> 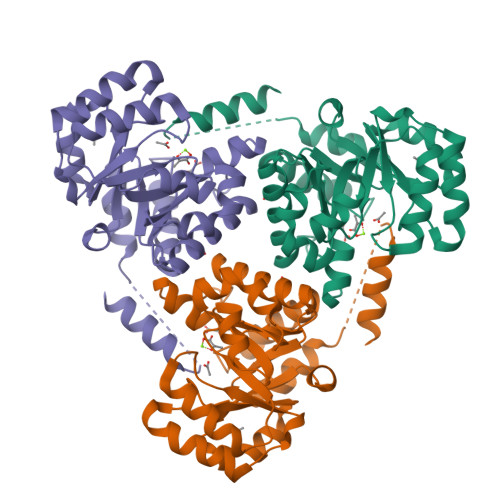MAHHHHHHMNLRAAGPGWLFCPADRPERFAKAAAAADVVILDLEDGVAEAQKPAARNALRDTPLDPERTVVRINAGGTADQARDLEALAGTAYTTVMLPKAESAAQVIELAPRDVIALVETARGAVCAAEIAAADPTVGMMWGAEDLIATLGGSSSRRADGAYRDVARHVRSTILLAASAFGRLALDAVHLDILDVEGLQEEARDAAAVGFDVTVCIHPSQIPVVRKAYRPSHEKLAWARRVLAASRSERGAFAFEGQMVDSPVLTHAETMLRRAGEATSE>[28x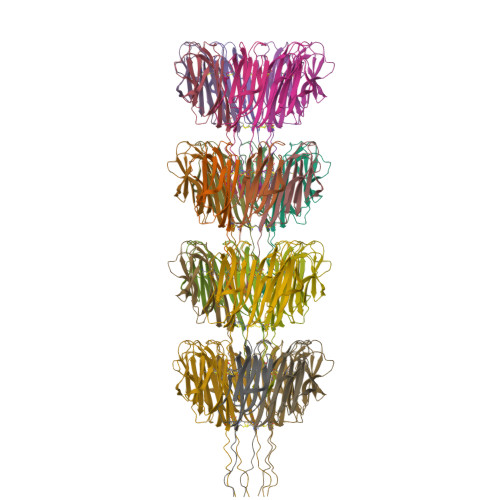]MAQIGNCCTEQLCCVNDAVCCTIILDDTGGTALPIWDDATTFVINGTIMVENNGTVGVGPTAALTVNGTAVGGFVVAPGECRSITMNDINSIAIVGAGTGTSSVKISFSINYKF> SPEDFYEVMRLIAVEILNADLEEAHKDQILAEFLNRHFSFSRTNGFSLKVKLEEQPQWINALGDFIQAVPERVDALVMSKLRPLLHYARAKDIDNYRTVEESYRQGQYYRFDIVDGKLNIQFNEGEPYFEGIDIAKPKVKMTAFKFDNHKIVTELTLNEFMIGEGHYDVRLKLHSRNKKHTMYVPLSVNANKQYRFNIMLEDIKAYLPKEKIWDVFLEVQIGTEVFEVRVGNQRNKYAYTAETSALIHLNNDFYRLTPYFTKDFNNISLYFTAITLTDSISMKLKGKNKIILTGLDRGYVFEEGMASVVLKDDMIMGMLSQTSENEVEILLSKDIKKRDFKNIVKLNTAHMTYSLK

In this article we describe the crystal structure of TarS, an enzyme responsible for the glycosylation of wall teichoic acid polymers of the S. aureus cell wall, a process that has been shown to be specifically responsible for methicillin resistance in MRSA. TarS possesses a catalytic domain with a canonical GTA fold (one of two distinct A/B folds characteristic of nucleotide-sugar dependent glycosyltransferases) consisting of two closely associated α/β/α sandwich Rossmann motifs that abut and form a continuous central β-sheet. TarS possesses a D(91)XDD motif with aspartates coordinating a metal cation, a feature that is typical of the GTA superfamily. Altogether, TarS features a novel architecture with closely-associated trimerization domains connected by a linker region to three protruding catalytic domains that face away from each other.

Limited (thermolysin) proteolysis of the purified full-length TarS protein resulted in crystals diffracting to ~ 2.3 Å resolution, with SAD phasing using an iodide derivative revealing cleavage of the N-terminal region of the catalytic domain (1–216) and the structure of the TarS217-573 as described. Two C-terminally localized regions in the TarS217-573 structure (encapsulating the trimerization domain), designated here as C1 (353–495) and C2 (496–573), were also observed, where a series of β-sheets of unique sequence participate in an extensive trimerization interface (buried surface area: 6970 Å2, predicted as stable by PISA) and connect to a linker composed of 2 anti-parallel β-strands and an α-helix that leads into the catalytic domain. Furthermore, prominent basic grooves along the surface of the trimerization domain, and notably along the C1 domain leading into the active site, suggest that both C1 and C2 domains likely participate in polyRboP binding. Another interesting feature is the close proximity (4.0 Å) of methionines (M521 and M532) from each of the 3 different monomers at the bottom surface of the trimerization interface, forming a hexameric methionine cluster that we hypothesize may be involved in promoting plasticity/adaptability of TarS during multivalent interactions with substrates or potential cell-wall partners. Furthermore, structure-guided mutants aimed at disrupting the trimerization interface (M521R, M532R) resulted in the expression of insoluble protein aggregates. The overlap of the TarS1-349 and TarS217-573 structures with regard to the C-terminus of the catalytic domain and the linker region (217–349) further allowed us to superimpose these domains relative to each other and to the lower resolution full-length structure, providing us with essentially high-resolution views for the entire span of the TarS structure. Given the prominent electropositive charge distribution along the surface of the TarS C1 and C2 domains leading into the active site, it is likely that both CBM domains may be involved in polyRboP binding.>MKIEEVKSTTKTQRIASHSHVKGLGLDESGLAKQAASGLVGQENAREACGVIVELIKSKKMAGRAVLLAGPPGTGKTALALAIAQELGSKVPFCPMVGSEVYSTEIKKTEVLMENFRRAIGLRIKETKEVYEGEVTELTPCETENPMGGYGKTISHVIIGLKTAKGTKQLKLDPSIFESLQKERVEAGDVIYIEANSGAVKRQGRCDTYATEFDLEAEEYVPLPKGDVHKKKEIIQDVTLHDLDVANARPQGGQDILSMMGQLMKPKKTEITDKLRGEINKVVNKYIDQGIAELVPGVLFVDEVHMLDIECFTYLHRALESSIAPIVIFASNRGNCVIRGTEDITSPHGIPLDLLDRVMIIRTMLYTPQEMKQIIKIRAQTEGINISEEALNHLGEIGTKTTLRYSVQLLTPANLLAKINGKDSIEKEHVEEISELFYDAKSSAKILADQQDKYMK[3x];>MATVTATTKVPEIRDVTRIERIGAHSHIRGLGLDDALEPRQASQGMVGQLAARRAAGVVLEMIREGKIAGRAVLIAGQPGTGKTAIAMGMAQALGPDTPFTAIAGSEIFSLEMSKTEALTQAFRRSIGVRIKEETEIIEGEVVEIQIDRPATGTGSKVGKLTLKTTEMETIYDLGTKMIESLTKDKVQAGDVITIDKATGKISKLGRSFTRARDYDAMGSQTKFVQCPDGELQKRKEVVHTVSLHEIDVINSRTQGFLALFSGDTGEIKSEVREQINAKVAEWREEGKAEIIPGVLFIDEVHMLDIESFSFLNRALESDMAPVLIMATNRGITRIRGTSYQSPHGIPIDLLDRLLIVSTTPYSEKDTKQILRIRCEEEDVEMSEDAYTVLTRIGLETSLRYAIQLITAASLVCRKRKGTEVQVDDIKRVYSLFLDESRSTQYMKEYQDAFLFNELKGETMDTS[3x]

R2TP (named after its components in yeast, Rvb1-Rvb2, Tah1 and Pih1) is an Heat shock protein 90 (HSP90) co-chaperone complex assembled from RuvB-like protein 1 (RUVBL1), RuvB-like protein 2 (RUVBL2), RNA polymerase–associated protein 3 (RPAP3), and PIH1 domain-containing protein 1 (PIH1D1) (1–5). RUVBL1 (Rvb1p in yeast) and RUVBL2 (Rvb2p in yeast) are essential and related AAA adenosine triphosphatases (ATPases), while PIH1D1 (Pih1p in yeast) is a client recruitment protein recognizing casein kinase 2 (CK2)–phosphorylated adaptors containing a consensus DpSDD/E motif. RUVBL1 and RUVBL2 assemble into heterohexameric rings with domain II (DII) from each subunit protruding from one face of the ring, while the other is defined by the ATPase domains. Here, we report cryo-EM structures of R2TP and show how access to the nucleotide-binding site of RUVBL2 is coupled to binding of the client recruitment component of R2TP (PIH1D1) to its DII domain.

To specifically explore the heterogeneity of the asymmetric “open” conformation of the RUVBL1-RUVBL2 ring, we reclassified the images using a mask focused on the open RUVBL2 subunit. 3D classification in three subgroups (71.8, 11.8, and 16.4% of the particles in each group) revealed two major conformations, which we then refined independently. Whereas the overall structure of the ring was similar to R2TP-ΔNT_structure, a much-pronounced distortion of the open RUVBL2 subunit was evident, accompanied by complete disappearance of regions corresponding to the N-terminal segment of RUVBL2 and ADP from the nucleotide-binding site. The rest of the subunits in the ring showed clear density for ADP. Thus, it appears that we have captured two conformations of a PIH1D1-bound complex, both inducing changes in the RUVBL2 subunit where PIH1D1 binds, but differing in the presence or absence of ADP bound to the open RUVBL2 subunit. The resolution in the open ADP-empty RUVBL2 subunit is lower than that in the rest of the complex, and we thus only considered the secondary-structure elements for model building. During model building, we found that the distorted rim of RUVBL2 corresponded to an N-terminal segment of RUVBL2 (residues 1 to 49), which was completely lost in the ADP-empty conformation. Comparison of the conformations of closed and open RUVBL2 subunits from the ADP-empty structure of R2TP-ΔNT, after alignment of their neighboring RUVBL1 subunits, reveals the motions in the context of the RUVBL1-RUVBL2 ring, and several major areas of change became apparent. First, changes in the position of several α helices suggest that the torsions of the DII-external domain accompanying its interaction with PIH1D1 are transmitted to the internal region of the DII domain, and this relays the changes to elements essential for nucleotide binding and nucleotide exchange.>AIAHLATEYVFSDFLLKEPTEPKFKGLRLELAVDKMVTCIAVGLPLLLISLAFAQEISIGTQISCFSPSSFSWRQAAFVDSYCWAAVQQKNSLQSESGNLPLWLHKFFPYILLLFAILLYLPPLFWRFAAAPHICSDLKFIMEELDKVYNRAIKAAKSARDLDMRDGACSVWSHPQFEKPGVTENLGQSLWEVSESHFKYPIVEQYLKTKKNSNNLIIKYISCRLLTLIIILLACIYLGYYFSLSSLSDEFVCSIKSGILRNDSTVPDQFQCKLIAVGIFQLLSVINLVVYVLLAPVVVYTLFVPFRQKTDVLKVYEILPTFDVLHFKSEGYNDLSLYNLFLEENISEVKSYKCLKVLENIKSSGQGIDPMLLLTNLGMIKMDVVDGKTPMSAEMREEQGNQTAELQGMNIDSETKANNGEKNARQRLLDSSC[7x]

Pannexin1 (PANX1) is a large-pore ATP efflux channel with a broad distribution, which allows the exchange of molecules and ions smaller than 1 kDa between the cytoplasm and extracellular space. Pannexin is a family of large-pore forming channels that play pivotal roles in cell-to-cell communication. Among the three isoforms of Pannexin (PANX1, PANX2, and PANX3), PANX1 is ubiquitously expressed in mammalian cells and has been extensively studied for its diverse activation modes, association with diverse signaling molecules and broad cellular and tissue distribution. The regulation of the PANX1 channel is complicated and remains unclear, but it is commonly accepted that PANX1 is regulated by extracellular potassium, intracellular calcium, ATP, mechanical stimuli, voltage, low oxygen stress, S-nitrosylation, and caspase cleavage.

To further elucidate the function of PANX1, we propose the full-length human Pannexin1 (hPANX1) model through cryo-electron microscopy (cryo-EM) and molecular dynamics (MD) simulation studies, establishing hPANX1 as a homo-heptamer and revealing that both the N-termini and C-termini protrude deeply into the channel pore funnel. Instead, we conducted extensive experiments and ultimately identified that residue V172—present in the intracellular linker domain—was suitable for inclusion of a Strep-tag; this linker domain was shown outside of the pore in previous structural studies. Single-particle analysis produced a 3D reconstruction of hPANX1 resolved at 3.15 Å under the gold-standard Fourier shell correlation criteria (FSC = 0.143), which was of sufficient quality to build models for the majority of protein regions. However, despite the confirmed presence of the full-length hPANX1 protein in the cryo sample, the electron densities accounting for the intracellular link (160–194) between TM2 and TM3 and the C-termini were subjected to local density falloff without local scaling and sharpening. We tentatively proposed the final structure as the hPANX1-MD model, which was generated based on the LocScale map and cMDFF-RSR modeling. In the resultant full-length hPANX1-MD model, the permeation pathway of the hPANX1 channel consists of an intracellular channel entrance, a pore funnel, and an extracellular cavity. The heptameric C-termini protrude deeply into the pore funnel and occupy the innermost layer. In particular, E414(422) and S424(432) formed major constrictions in the channel at the intra-cellular and extra-cellular ends respectively; the intracellular constriction was abruptly enlarged at N412(420) through a turn at G413(421). Thus, our current hPANX1 model is in a closed state.> MVRGIRGAITVNSDTPTSIIIATILLLEKMLEANGIQSYEELAAVIFTVTEDLTSAFPAEAARQIGMHRVPLLSAREVPVPGSLPRVIRVLALWNTD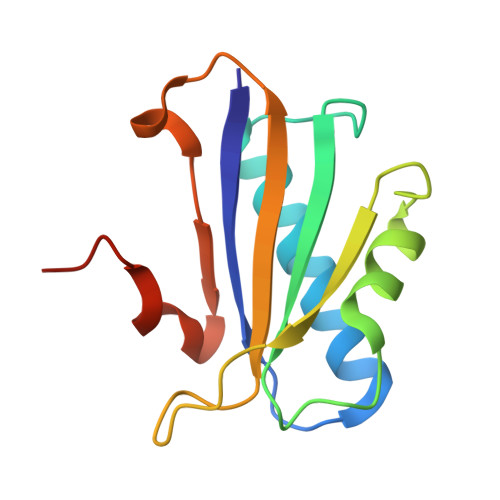TPQDRVRHVYLSEAVRLRPDLESAQL>MSSQIYIPDLLITWPWQKVRNPLLQEVQDEANEWVKSFVLFEPEQFEKFKACDFNLLGALVGPLGTKEELRISCDLMNFYFAFDEYTDLASADEAKVIARDVMESFRHTDKPSHNKITEMARQFFERTINTVGNDPTGIEQFIADFDAYTTSIIQEADDRASGHIRSVEDYFILRRDTCGGKPSFSFFGLGLNIPKEVFAHPMFISMTESATDLIAITNDMHSYNLEQSRGLDGHNVITAIMHEYKINLQGALYWLSGYATKTIAKFISDRKNLPSWGPVVDRAVEQYFDRVGRCVRGYDAWSYETKR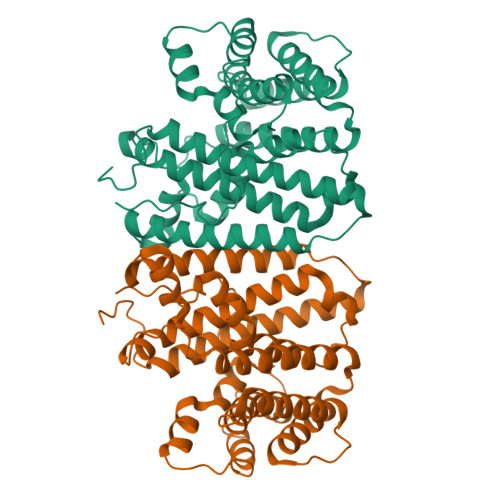YYGKNGLEIQKTRQITL[2x]> VFKKVLLTGTSEESFTAAADDAIDRAEDTLDNVVWAEVVD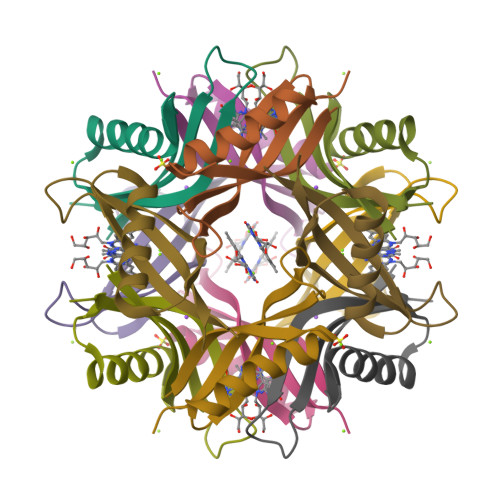QGVEIGAVEERTYQTEVQVAFELD> MSTMSTPAAEQRKLVEQLMGRDFSFRHNRYSHQKRDLGLHDPKICKSYLVGECPYDLFQGTKQSLGKCPQMHLTKHKIQYEREVKQGKTFPEFEREYLAILSRFVNECNGQISVALQNLKHTAEERMK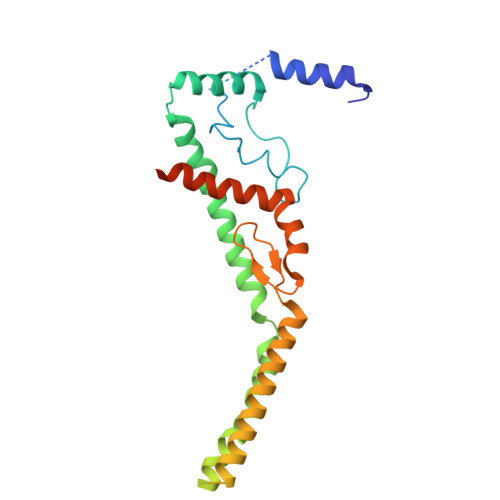IQQVTEELDVLDVRIGLMGQEIDSLIRADEVSMGMLQSVKLQELISKRKEVAKRVRNITENVGQSAQQKLQVCEVCGAYLSRLDTDRRLADHFLGKIHLGYVKMREDYDRLMKNNRTTNASKTATTLPGRRFV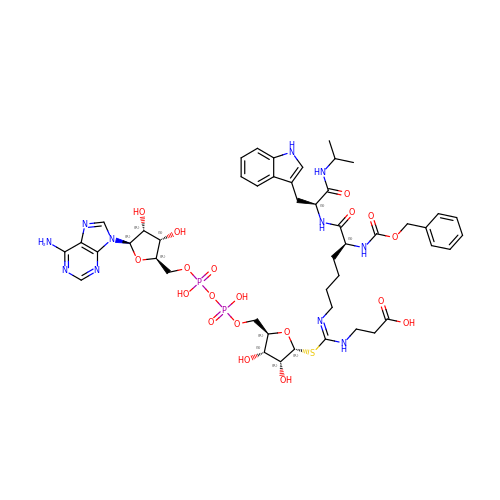3-[[(~{Z})-~{C}-[(2~{R},3~{R},4~{S},5~{R})-5-[[[[(2~{R},3~{S},4~{R},5~{R})-5-(6-aminopurin-9-yl)-3,4-bis(oxidanyl)oxolan-2-yl]methoxy-oxidanyl-phosphoryl]oxy-oxidanyl-phosphoryl]oxymethyl]-3,4-bis(oxidanyl)oxolan-2-yl]sulfanyl-~{N}-[(5~{S})-6-[[(2~{S})-3-(1~{H}-indol-3-yl)-1-oxidanylidene-1-(propan-2-ylamino)propan-2-yl]amino]-6-oxidanylidene-5-(phenylmethoxycarbonylamino)hexyl]carbonimidoyl]amino]propanoic acid | C47 H63 N11 O19 P2 S | GGZPCSBRGOFORP-PVLZSEPSSA-N VAMP7 (also termed Ti-VAMP) (Advani et al., 1998; Galli et al., 1998) is one of the largest R-SNAREs, having a 120 residue N-terminal longin domain (Pryor et al., 2008; Rossi et al., 2004). It is involved in the fusion of lysosomes, late endosomes, and compartments derived from them with a number of target membranes including the plasma membrane and endosomes (for a comprehensive review of VAMP7 function see (Chaineau et al., 2009)). AP3 (subunits δ, β3, μ3, σ3) is one of the family of heterotetrameric clathrin adaptors that in mammalian cells has been localized mainly to tubulovesicular, early-sorting/recycling endosomes with a minor location at the trans-Golgi network (TGN) (Peden et al., 2004; Simpson et al., 1996; Theos et al., 2005). We show that the linker of the δ-adaptin subunit of AP3 binds the VAMP7 longin domain and determines the structure of their complex.

Crystals of this construct showed anisotropic diffraction to 2.8 Å in the best direction. The structure of the complex was readily solved by molecular replacement using as the search model the longin domain only of VAMP7 extracted from the Hrb/VAMP7 longin domain structure (Pryor et al., 2008). This showed two molecules in the asymmetric unit. The two copies in the asymmetric unit, which represent the VAMP7 longin domain/δ-adaptin complex (i.e., excluding the connection arising from the fusion protein) are very similar in structure despite their different crystal environments, showing that the structure is not perturbed in the fusion protein construct. Surprisingly, since there is no detectable sequence homology between the relevant portions of Hrb and δ-adaptin, the fragment of δ-adaptin binds to the longin domain following approximately the same route as that taken by Hrb (Pryor et al., 2008) and by VAMP7's own SNARE motif (as inferred from biochemical [Pryor et al., 2008] and NMR shift mapping [Vivona et al., 2010]). This δ-adaptin/Hrb binding site is a hydrophobic trough that runs half way round the VAMP7 longin domain. The interaction buries a total of around 1,990 Å2 of solvent accessible surface area (determined with PISA; Krissinel and Henrick, 2007) and is mediated by mainly hydrophobic residues, which is typical of the low μM KD interactions seen in the protein:protein interactions involved in transport vesicle formation. The corresponding interface on the VAMP7 longin domain includes Leu4, Phe25, Val28, Ile32, Lys42, Leu43, Tyr45, Tyr50, and Phe52.

>[2x]GSPFYIKSSPSPQKRYQDTPGVEHIPVVQIDLSVPLKVPGLPMSDQYVKLEEAMAILFAVVARGTTILAKHAWCGGNFLEVTEQILAKIPSENNKLTYSHGNYLFHYICQDRIVYLCITDDDFERSRAFSFLNEVKKRFQTTYGSRAQTALPYAMNSEFSSVLAAQLKHHSEN>MGSSHHHHHHSSGLVPRGSHSQPSTANGGFPSVVVTAVTATTSISPDIESTWKGLLAGESGIHALEDEFVTKWDLAVKIGGHLKDPVDSHMGRLDMRRMSYVQRMGKLLGGQLWESAGSPEVDPDRFAVVVGTGLGGAERIVESYDLMNAGGPRKVSPLAVQMIMPNGAAAVIGLQLGARAGVMTPVSACSSGSEAIAHAWRQIVMGDADVAVCGGVEGPIEALPIAAFSMMRAMSTRNDEPERASRPFDKDRDGFVFGEAGALMLIETEEHAKARGAKPLARL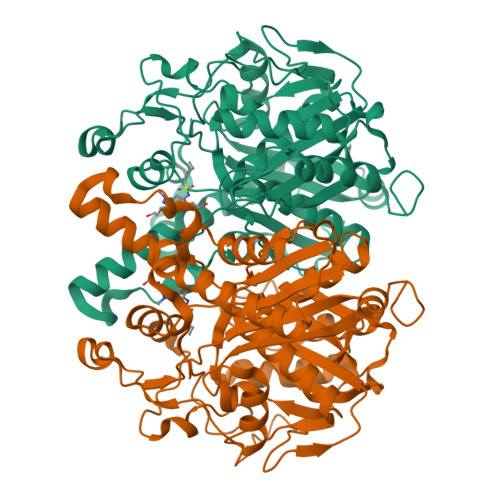LGAGITSDAFHMVAPAADGVRAGRAMTRSLELAGLSPADIDHVNAHGTATPIGDAAEANAIRVAGCDQAAVYAPKSALGHSIGAVGALESVLTVLTLRDGVIPPTLNYETPDPEIDLDVVAGEPRYGDYRYAVNNSFGFGGHNVALAFGRY[2x]8-fluoro-2-(3-piperidin-1-ylpropanoyl)-1,3,4,5-tetrahydrobenzo[c][1,6]naphthyridin-6(2H)-one | C20 H24 F N3 O2 | 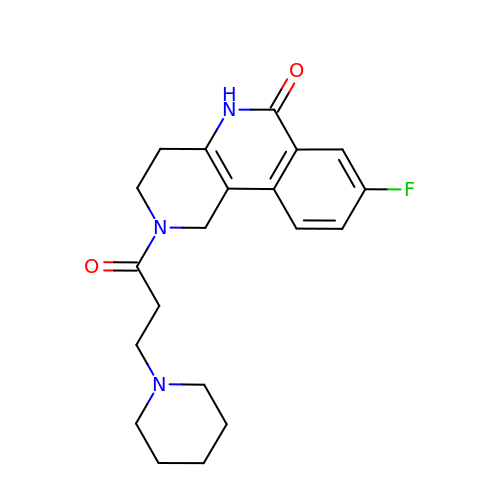CTOQXIXQHAILCA-UHFFFAOYSA-N> GPLGSGKKCYKLENEKLFEEFLELCKMQTADHPEVVPFLYNRQQRA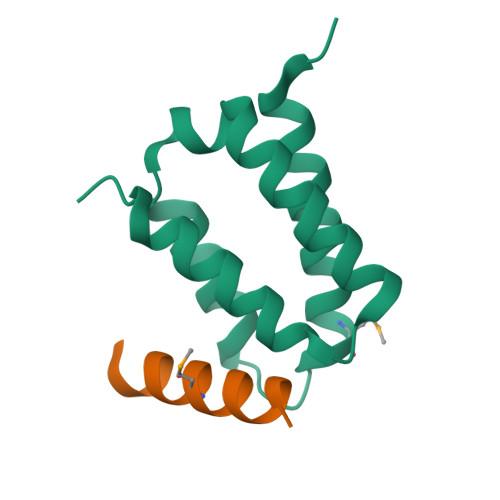HSLFLASAEFCNILSRVLSRARSRPAKLYVYINELCTVLKAHSAKKKLN;> SENRIAKKMLLEEIKANLSSDED>GMLKIGVIADDFTGATDIASFLVENGMPTVQINDVPTGTQPEGCDAVVISLKTRSCPAQEAIKQSLAALVWLKKQGCQQVYFKYCSTFDSTAEGNIGPVTDALMVALDTSFTVISPALPVNGRTVYQGYLFVMNHLLAESGMRHHPINPMTDSYLPRLMEAQAQGRCGVIPAQTLDEGVAATRAALSRLQQEGYRYAVLDALNERHLEIQGEVLRDAPLVTGGSGLAMGLARQWAKHGVSQARSAGYPLSGRAVVLSGSCSQMTNQQVAFYRQHAPTRDVDVARCLSSETREAYAEALAQWVLSQDSELAPMI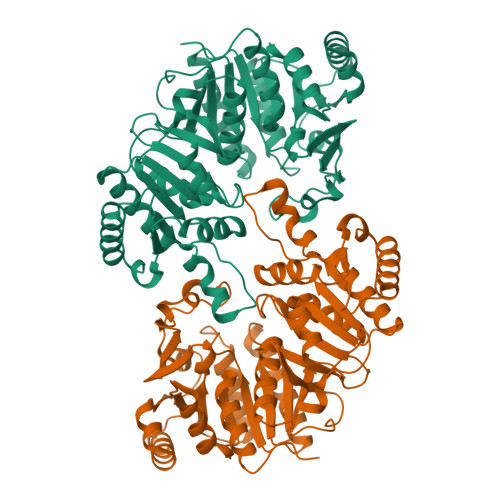SATASTQALAAIQQQYGATEASHAVEALFSLLAARLAEGGITRFIVAGGETSGVVTQSLGITGFHIGPCISPGVPWVNALHAPVSLALKSGNFGDESFFIRAQREFQV[2x]>MGTESGSDPESSSNGWSRARGLVVKTLVLIGGALLIKRLTKSTTRRDHARV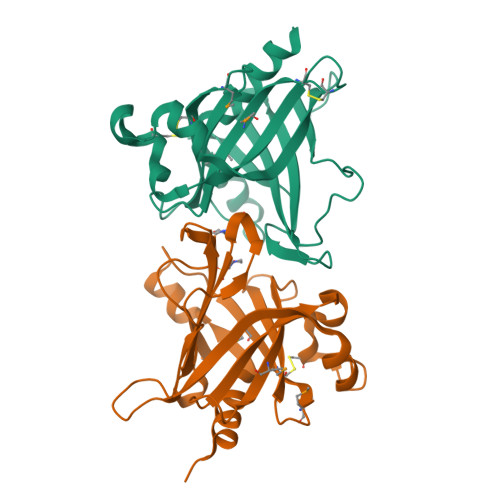VSRSLTGEKFTREQASRDPDNYFNIRMLSCPAAEMVDGSEVLYLEQAFWRTPQKPFRQRLYMVKPCPKELKCDVEVSSYAIRDAEEYKNFCDRPKDQRPLPEEVIGDIGEHLTTIHLNCCDRGKRCLYEGSTSPGGFPNSWNGASYCTSDLAVLKNNEIHLWDRGFDENRNQVWGPKEGPYEFKPATSSSINENLSALNILYQSSIDKPIQGSLILQD[2x]> ASVGGSLTGVGSIVTCLDSGRPGSIPCSKKWVLTLAVENGATAASSSVSATQAVYGSSSANATVRSADNPNTVYAFKYQVHITLTKSRIRLDYPLYYQSDFNNKPYEIVYKYNQKGPLNWLDNQCVATWGSSDPTCGYAYNPSWSTKPADRILYSQGFCCDCNAGDLLGLSPNRIRGGLDCSLLNFDNPTESAHCLRFDSLWYSAFQIGEPDVNFVILVNVTKCPLANSTIKSISGLVGNQDQAIQNCSTEIISLSPSSPIGYASNGKISAQAIGDFAPWEGTPSYSEKLFFVPSVCTDTSEAWCVDRISY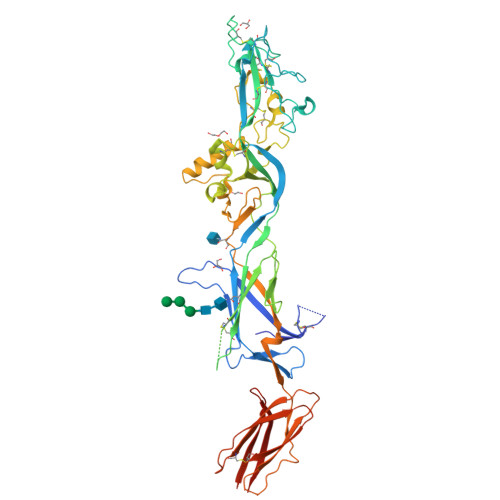IPTEINRWMLIDNDLVTITGDTCDKIGVSYSAFTNEGQRCERPTQSCLHDQLQDYYDSDLALEQTGKVGSYFVQFFGDFDVSGLTPRNPLLRFFTNRTQATEVVLQFAAEELFYTIYLAPARFLRHLSKINPFTSQSKGGLIDLWIVSEGTGQNAAQFTVSASCEPNVEPIQAQIVTLAPGQLVSISLPIIETKATGGAGVCNCTLRNALGQVLDVLVLEFNASSVHHHHHHHH> KILKKQELCKNLVAQGMNGYQHITLPNWVCTAFHESSYNTRATNHNTDGSTDYGILQINSRYWCHDGKTPGSKNACNISCSKLLDDDITDD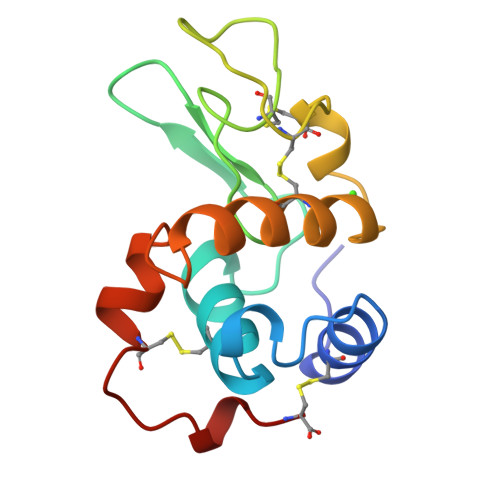LKCAKKIAGEAKGLTPWVAWKSKCRGHDLSKFKC> GSHMDAFDTLFDHAPDKLNVVKKTLITFVNKHLNKLNLEVTELETQFADG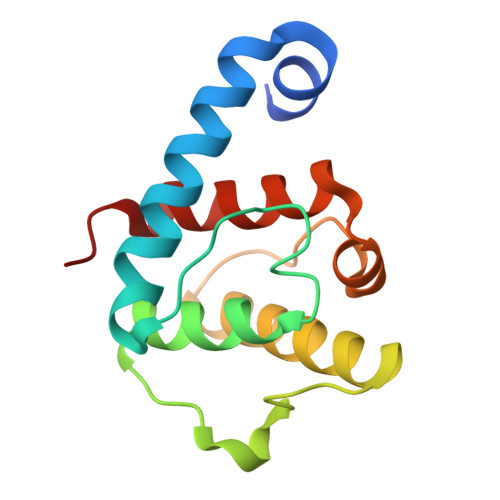VYLVLLMGLLEGYFVPLHSFFLTPDSFEQKVLNVSFAFELMQDGGLEKPKPRPEDIVNCDLKSTLRVLYNLFTKYRNVE>MVRVTTNPVDLWSAPSSQARLEKEYFDQHFGPFFRTEQLIIRAPLTDKHIYQPYPSGADVPFGPPLDIQILHQVLDLQIAIENITASYDNETVTLQDICLAPLSPYNTNCTILSVLNYFQNSHSVLDHKKGDDFFVYADYHTHFLYCVRAPASLNDTSLLHDPCLGTFGGPVFPWLVLGGYDDQNYNNATALVITFPVNNYYNDTEKLQRAQAWEKEFINFVKNYKNPNLTISFTAERSIEDELNRESDSDVLEHHHHHHHH[2x]

Niemann–Pick C1 protein (NPC1) is a membrane protein that primarily resides in late endosomes and lysosomes, and plays an important role in cholesterol homeostasis in the cell. NPC1 is a 13-pass transmembrane glycoprotein that resides primarily in late endosomes and lysosomes. The second luminal domain of NPC1 (NPC1-C) serves as the intracellular receptor for Ebola and Marburg viruses. The viral glycoprotein (GP) interacts with domain C of NPC1 (termed NPC1-C here), which is one of three large luminal loops of the protein.

The goal was to co-crystallize NPC1-C in complex with primed A82V Ebola virus glycoprotein (GP) as part of an effort to explore the basis of the enhanced infectivity of the A82V variant in the 2013–2016 Ebola outbreak in West Africa. Human NPC1-C (residues 371–621) was expressed as a C-terminally polyhistidine-tagged fusion protein in E. coli as insoluble inclusion bodies. After denaturation with urea and a nickel-affinity chromatography step, the protein was refolded at pH 8 using the glutathione redox system to facilitate correct disulfide-bond formation. Although the objective was to obtain a crystal of a protein complex of NPC1-C with the primed and glycosylated form of A82V EBOV GP, the proteins did not co-crystallize regardless of the glycosylation state of NPC1-C, with nonglycosylated NPC1-C crystallizing alone. The two disulfide bonds that were expected in the structure, i.e. Cys468–Cys479 and Cys516–Cys533, are clearly resolved in the electron density, indicating that the refolding protocol was effective. In full-length NPC1, domains C and I fold into similar structures, intertwine with each other through an extensive interface and form a tunnel that may function as a path for cholesterol transfer. It is likely that the absence of domain I allowed NPC1-C to crystallize as dimers using the same domain I packing interface. The overall structure of NPC1-C is similar to other published structures of NPC1, as expected, with root-mean-square deviations on all common Cα atoms for each aligned pair ranging from 0.36 to 0.78 Å. NPC1-C uses these loops to engage with its binding partners, explaining the different configurations.>STSAGPTVPDRDNDGIPDSLEVEGYTVDVKNKRTFLSPWISNIHEKKGLTKYKSSPEKWSTASDPYSDFEKVTGRIDKNVSPEARHPLVAAYPIVHVDMENIILSKNEDQSTQNTDSQTRTISKNTSTSRTHTSEPGSNSNSSTVAIDHSLSLAGERTWAETMGLNTADTARLNANIRYVNTGTAPIYNVLPTTSLVLGKNQTLATIKAKENQLSQILAPNNYYPSKNLAPIALNAQDDFSSTPITMNYNQFLELEKTKQLRLDTDQVYGNIATYNFENGRVRVDTGSNWSEVLPQIQETTARIIFNGKDLNLVERRIAAVNPSDPLETTKPDMTLKEALKIAFGFNEPNGNLQYQGKDITEFDFNFDQQTSQNIKNQLAELNATNIYTVLDKIKLNAKMNILIRDKRFHYDRNNIAVGADESVVKEAHREVINSSTEGLLLNIDKDIRKILSGYIVEIEDTEGLKEVINDRYDMLNISSLRQDGKTFIDFKKYNDKLPLYISNPNYKVNVYAVTKENTIINPSENGDTSTNGIKKILIFSKKGYEIG[4x];>AGGHG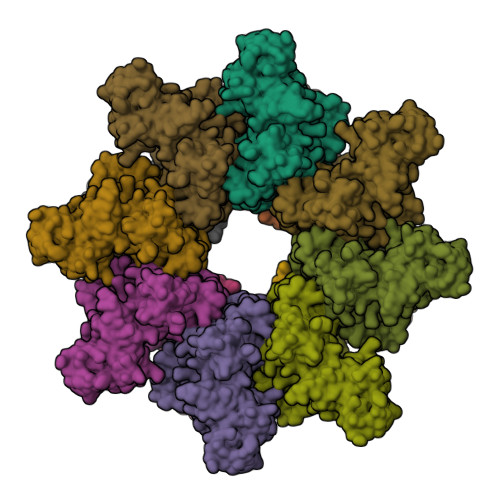DVGMHVKEKEKNKDENKRKDEERNKTQEEHLKEIMKHIVKIEVKGEEAVKKEAAEKLLEKVPSDVLEMYKAIGGKIYIVDGDITKHISLEALSEDKKKIKDIYGKDALLHEHYVYAKEGYEPVLVIQSSEDYVENTEKALNVYYEIGKILSRDILSKINQPYQKFLDVLNTIKNASDSDGQDLLFTNQLKEHPTDFSVEFLEQNSNEVQEVFAKAFAYYIEPQHRDVLQLYAPEAFNYMDKFNEQEINLSLEELKDQR[2x]Vibrio bacteria require iron for growth and survival. They utilize a ferric ion‐binding protein (FbpA) to bind and transport Fe3+ into the cell. Most gram‐negative bacteria contain the highly conserved FbpA protein, which is considered bacterial transferrin and binds to free Fe3+. Therefore, FbpA can bind Fe3+ in the periplasm of gram‐negative bacteria and transport it intracellularly through a transmembrane channel while consuming ATP during transport (Lu et al. 2019). FbpA from Vibrio metschnikovii (Vm) is a potential target for inhibiting its growth.

Diffraction‐quality crystals of RA‐treated VmFbpA were obtained with a reservoir composition of 1 M (NH4)2HPO4 and 0.1 M imidazole‐HCl (pH 8.0). However, in the crystal structure, only a partial electron density of RA was observed at the Fe3+‐binding site. The RPC results indicated that the binding with VmFbpA was a degradation product of RA, DSS. Therefore, despite RA and VmFbpA being used for co‐crystallization, only the degradation product of RA was observed. Compared with Fe3+‐bound VmFbpA, DSS‐bound VmFbpA underwent a 2.1° rotation in its N‐lobe; however, compared with apo VmFbpA, the protein did not undergo any significant conformational changes. In the ligand binding region, DSS bound to VmFbpA through hydrophobic interactions and hydrogen bonds. Gln58, Asn138, and Asn193 directly interacted with DSS through hydrogen bonding, including the O10 of DSS–Nε2 of Gln58, O of H2O (443)–Oε1 of Gln58, O of H2O (443)–O10 of DSS, O13 of DSS–Nδ2 of Asn138, and O13 of DSS–Nδ2 of Asn193. Interestingly, Arg199 did not directly interact with DSS, but instead, interacted with one hydroxyl group (O14) of DSS through a H2O (444). O of H2O (444) formed hydrogen bonds with both Nη2 of Arg199 and O14 of DSS, thereby stabilizing the binding of DSS to VmFbpA. When DSS binds, DSS sterically clashes with the Asn193 in the apo conformation, forcing it into a new conformation.

> QDITLYSGRGETLVKPIIEQFEKQSGIKVNVRYGDTAQLAVLLQEEGARSPADVYWGQDAGAMGALANAGLLATLPEAVYKQLPEIYTSKTGQWVAASGRSRVIAYSTERASAEDIPASVFDLTSEKYQGRFGLAPTNGGFQSFVTAMRVQHGDEKTLAWLKAMKANQPKIYRNNTTQIQAIGDGEIDFALVNNYYLPRFVAANASFPAKQTYFAEGDIGNLVNVAGVAVLKSSKKQPQAIQFIEYMLSPAAQQYFTSVVGEYPVTQGIIPNPVLGELDTLLQAAPSIDLDQLADLQGTLKLLRDAGLL> MSAGINYVQNYNGNLGDFTYDESAGTFSMYWEDGVSSNFVVGLGWTTGSSNAITYSAEYSASGSSSYLAVYGWVNYPQAEYYIVEDYGDYNPCSSATSLGTVYSDGSTYQ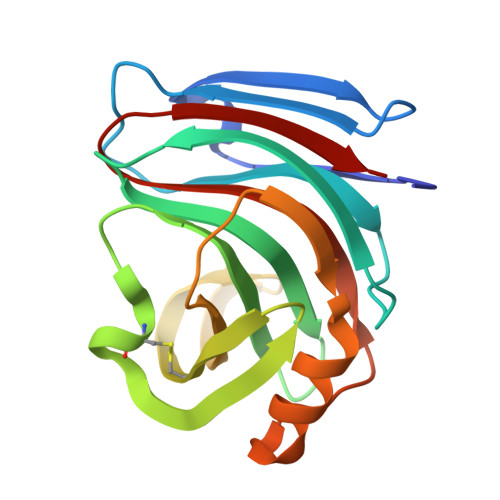VCTDTRTNEPSITGTSTFTQYFSVRESTRTSGTVTVANHFNFWAQHGFGNSDFNYQVMAVEAWSGAGSASVTISS> MNPPTFSPALLVVTEGDNATFTCSFSNTSESFVLNWYRMSPSNQPDKLAAFPEDRSQPGQDSRFRVTQLPNGRDFHM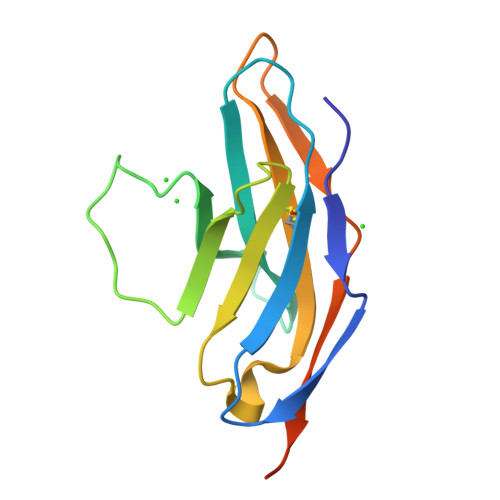SVVRARRNDSGTYLCGAISLAPKVQIKESLRAELRVTERRAEGSWSHPQFEK Nine new crystal structures of CG-rich DNA 18-mers with the sequence 5′-GGTGGGGGC-XZ-GCCCCACC-3′, which are related to the bacterial repetitive extragenic palindromes, are reported. All 18-mers crystallized as isomorphic tetragonal crystals with one strand of a right-handed antiparallel duplex in the asymmetric unit. All reported structures co-crystallized with the Sr2+ cation located between nucleotides 6 and 7 and (by symmetry) 12 and 13.

Of the four YY 18-mers, only Chom-18-CT could not be crystallized. Both Chom-18-TC and Chom-18-CC have high propeller twist; its extreme value in Chom-18-CC precludes assignment of the base-pair category. When we measure the distances between the C1′ atom of nucleotide 9 and C1′ of its symmetry-related base-paired nucleotide 10 in all 18-mers, the order from the shortest to the longest is TT (7.9 Å) < CC < TC < GT < GC < AC < AT < TA < CG < AG (12.1 Å). This trend follows the size of the pyrimidine–pyrimidine (Y–Y), pyrimidine–purine (Y–R/R–Y) and purine–purine (R–R) pairs regardless of the type of base pair involved.

> GGTGGGGCCCGCCCCACC> MDIIFVCTGNTCRSPMAEALFKSI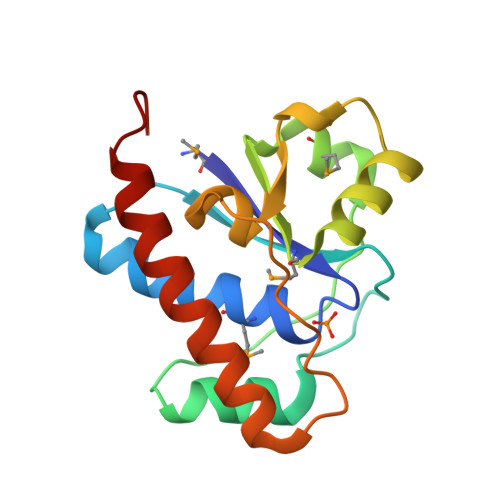AEREGLNVNVRSAGVFASPNGKATPHAVEALFEKHIALNHVSSPLTEELMESADLVLAMTHQHKQIIASQFGRYRDKVFTLKEYVTGSHGDVLDPFGGSIDIYKQTRDELEELLRQLAKQLKKDRRL O-(ADENOSINE-5'-O-YL)-N-(L-TYROSYL)PHOSPHORAMIDATE 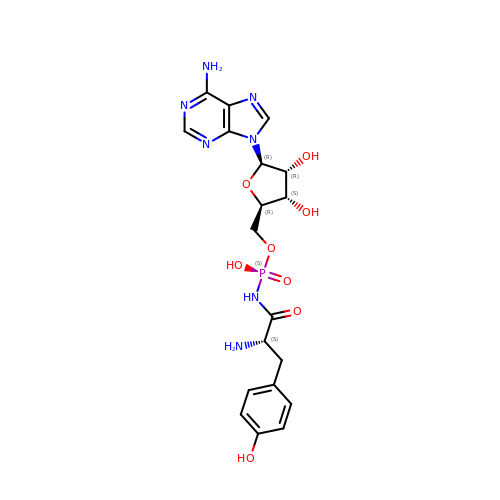| C19 H24 N7 O8 P | WJKRKCCMHCWYJU-QTOWJTHWSA-N>MYDVTEWKHVFKLDPNKDLPDEQLEILCESGTDAVIIGGSDGVTEDNVLRMMSKVRRFLVPCVLEVSAIEAIVPGFDLYFIPSVLNSKNADWIVGMHQKAMKEYGELMSMEEIVAEGYCIANPDCKAAALTEADADLNMDDIVAYARVSELLQLPIFYLEYSGVLGD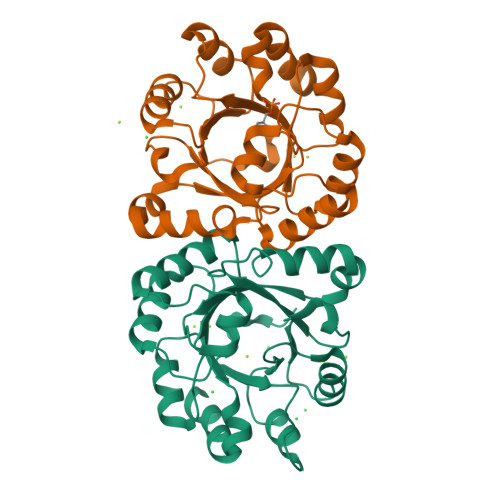IEAVKKTKAVLETSTLFYGGGIKDAETAKQYAEHADVIVVGNAVYEDFDRALKTVAAVKGE[2x]> DSDLQKALKKACSVEETAPKRKHVRACIVYTWDHQSSKAVFTTLKTLPLANDEVQLFKMLIVL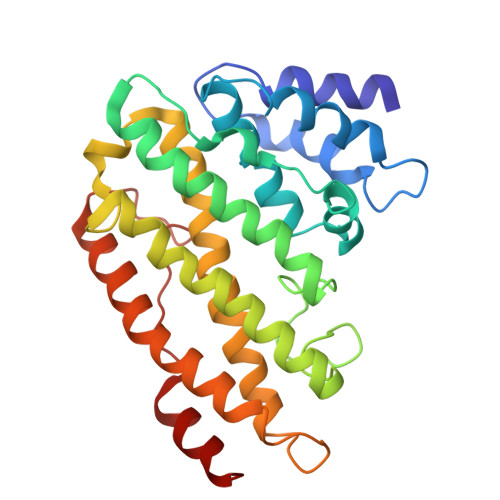HKIIQEGHPSALAEAIRDRDWIRSLGRVHSGGSSYSKLIREYVRYLVLKLDFHAHHRGFNNGTFEYEEYVSLVSVSDPDEGYETILDLMSLQDSLDEFSQIIFASIQSERRNTECKISALIPLIAESYGIYKFITSMLRAMHRQLNDAEGDAALQPLKERYELQHARLFEFYADCSSVKYLTTLVTIPKLPVDAPDVFLINDVDE>[2x]GSMPVVINSFNYDDPVNDNTIIYIRPPYYETSNTYFKAFQIMDNVWIIPERYRLGIDPSLFNPPVSLKAGSDGYFDPNYLSTNTEKNKYL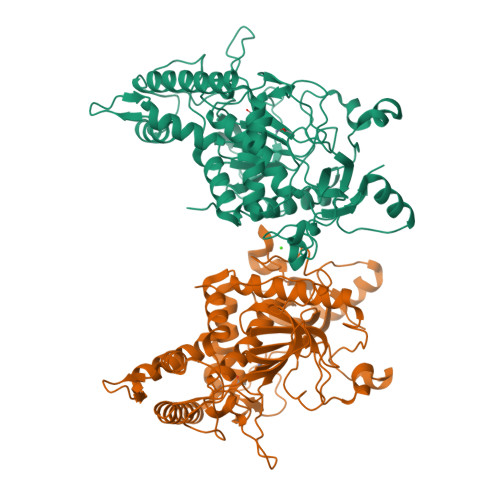QIMIKLFKRINSKPAGQILLEEIKNAIPYLGNSYTQEEQFTTNNRTVSFNVKLANGNIVQQMANLIIWGPGPDLTTNKTGGIIYSPYQSMEATPYKDGFGSIMTVEFSPEYATAFNDISIASHSPSLFIKDPALILMHELIHVLHGLYGTYITEYKITPNVVQSYMKVTKPITSAEFLTFGGRDRNIVPQSIQSQLYNKVLSDYKRIASRLNKVNTATALINIDEFKNLYEWKYQFAKDSNGVYSVDLNKFEQLYKKIYSFTEFNLAYEFKIKTRLGYLAENFGPFYLPNLLDDSIYTEVDGFNIGALSINYQGQNIGSDINSIKKLQGQGVVSRVVRLCSNSNTK> IVGGTEVEEGEWPWQASLQWDGSHRCGATLINATWLVSAAHCFTTYKNPARWTASFGVTIKPSKMKRGLRRIIVHEKYKHPSHDYDISLAELSSPVPYTNAVHRVCLPDASYEFQPGDVMFVTGFGALKNDGYSQNHLRQAQVTLIDATTCNEPQAYNDAITPRMLCAGSLEGKTDACQGD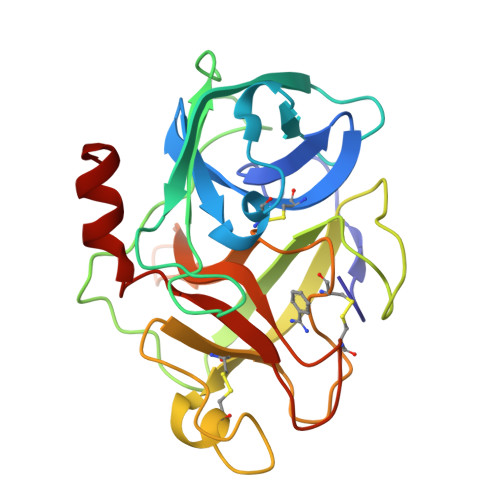SGGPLVSSDARDIWYLAGIVSWGDECAKPNKPGVYTRVTALRDWITSKTGI SPH1118 has been identified as a pectin-binding protein involved in both pectin chemotaxis and assimilation. SPH1118 shows high homology with the solute-binding protein (SBP) associated with the bacterial ABC transporter. SPH1118 consisted of two domains with a large cleft between the domains and substrates bound to positively charged and aromatic residues in the cleft through hydrogen bond and stacking interactions. Here we show tertiary structures of SPH1118 with six different conformations as determined by X-ray crystallography.

The space group of this crystal was C2221. One molecule was included in the asymmetric unit of the crystal. Residues 1 and 611–619 were unable to be assigned because of the poor electron density map. SPH1118 consisted of 21 α-helices and 5 β-sheets built from 15 β-strands. The C terminus of the C terminal domain (residues 573–610, Fig. 2a cyan) in SPH1118 formed a small additional domain and was located in the direction of the N terminal domain. SPH1118 is the first example of SBP in cluster C that binds to polysaccharide such as pectin. The surface electrostatic potentials of SPH1118 calculated at pH 7.0 showed that the cleft between the two domains was positively charged. Interestingly, SPH1118 showed three conformations [SPH1118 (open form), SPH1118 (full open form), and SPH1118 (closed form)] even in the substrate-free state. The crystallization conditions of SPH1118 (open form), SPH1118 (full open form), and SPH1118 (closed form) contained the substrates (ΔtriGalUA or sodium PG). However, no substrates were bound to SPH1118 in these structures. Compared to the C terminal domain of SPH1118 (full open form), those of SPH1118 (open form) and SPH1118 (closed form) were closed by 18.9° and 34.2°, respectively, suggesting that the domain of SPH1118 was flexibly opened and closed even in the substrate-free state. The crystal structures of SPH1118 (full open form) and SPH1118 (closed form) were obtained only under crystallization conditions in the presence of sodium PG. Conversely, the crystal structure of SPH1118 (open form) was obtained under several different conditions other than those shown in Supplementary Table 2, indicating that SPH1118 (open form) was likely to have a more stable conformation than any other substrate-free conformation.

> AFTQAPMLEQNKQLPPVDQRLPEKPLVIKPIASNGVYGGTLRTVMRGNADGNGILRTIGPQGLTHWTQDIQTVEPYVAESYTVSPDAMEYTFKLRKGMKWSDGTPFTADDIVFAMNDVVLNKEMFPQTPSAYLVGGKAPKVSKVDDYTVKFEFPAANLSFPETLATPLGQHPTLYQKKYCSQFHPAYNKNVQAEFTKANVKDWPSLMRAKCSDIELPSRWSSTERPSIDPWLIKEPYGGAVTRVVMERNPFYWQVDPTGKQLPYVDRIQYAVVSDLQAIILAATNGQYDIEARLLGSDVTSRPLMLKNQQKGGYKVFGQTSANANAAGLWLNQTTKNEKLRKYMTQHDFRQALSLAMDRDEINKVAWLGQAAPWQSGPFKESKWYNEKLATQYLKLDLAQANQILDRLGLTKRDSDGYRTYPDGGRVSLDAIVMIDRQAMVQTLELIRRQWQKAGVELVIKGSERSLFYNRATANDYDISIDVFPGGLDATLNPRAYVAVHPLESRMSLEWAKWYLSGGKQGIEPNESMKKRMALYDQFVAAKTQSQALSLFKQILQISADEFEVIGTVRPAVISSLHSLKLQNVNEKMPFGWPYATPSLSLPQQWYFS2-(4-fluorophenyl)-6-methyl-3-(pyridin-4-yl)pyrazolo[1,5-a]pyridine | C19 H14 F N3 | 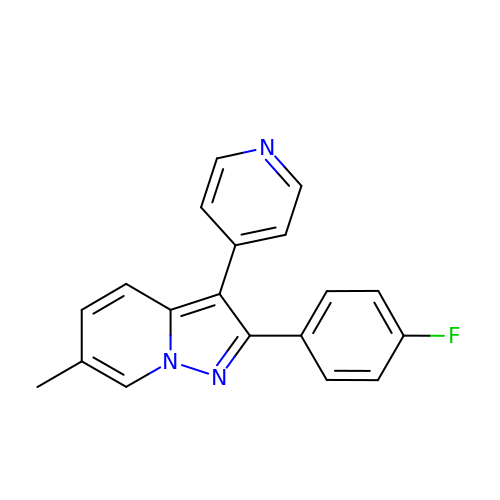DLJKUEGEDDMTMQ-UHFFFAOYSA-N>MFRTEDQSALRVGTDGIYPPHSFHAQDGRGELTGFDIDLIKEVAHRLNLKVEFFETAVSGLITGLDTNRYDVLVNVAITPERQKKYDFSIPYIAHRVLLVVRSDQQDIRSFKDLTDKTVAQILGTDLSRFAKELKSHLVFSHNFEQSLQLLLSKRTDATMIPDIPFFNFLERRPH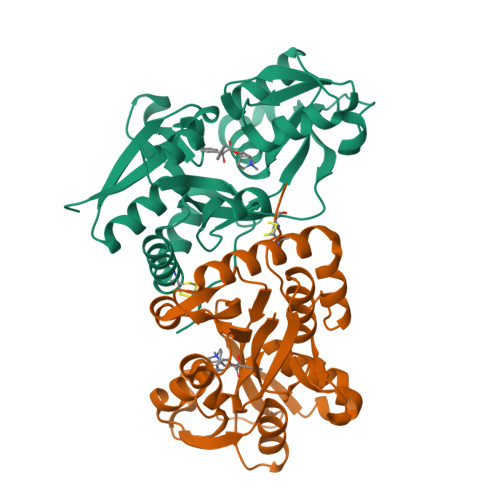DGNLFKIADRMKDNSAVAFMMRKGNNKLTRSINEILCAIHLDGTYKKIFDRYFDKNIISSVPGCSS[2x]>[8x]MSQQPGVLPENMKRYMGRDAQRMNILAGRIIAETVRSTLGPKGMDKMLVDDLGDVVVTNDGVTILREMSVEHPAAKMLIEVAKTQEKEVGDGTTTAVVVAGELLRKAEELLDQNVHPTIVVKGYQAAAQKAQELLKTIAMEVGAQDKEILTKIAMTSITGKGAEKAKEKLAEIIVEAVSAVVDDEGKVDKDLIKIEKKSGASIDDTELIKGVLVDKERVSAQMPKKVTDAKIALLNEAIEIKETETDAEIRITDPAKLMEFIEQEEKMLKDMVAEIKASGANVLFVQKGIDDLAQHYLAKEGIMAARRVKKSDMEKLAKATGANVITNIKDLSAQDLGDAGLVEERKISGDSMIFVEEVKH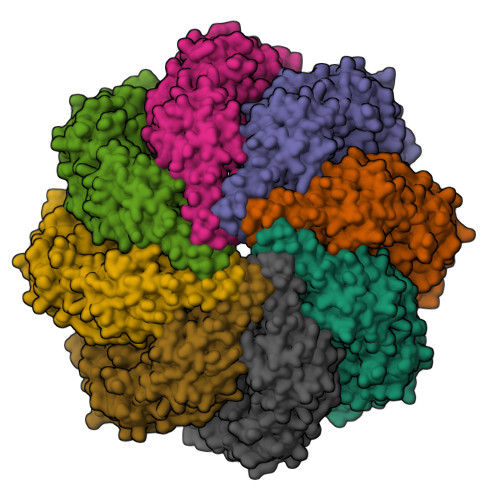PKAVTMLIRGTTEHVIEEVARAVDDAVGVVGSTIEDGRIVSGGGSTEVELSMKLREYAEGISGREQLAVRAFADALEVIPRTLAENAGLDAIEILVKVRAAHASNGNKYAGLNVFTGAVEDMTENGVVEPLRVKTQAIQSAAESTEMLLRIDDVIAAEKLRGAPDMGDMGGMPGMGGMPGMM>MKLTGKQTWEFENPLFVNSSGTAVGPKEKEGPLGHLFDKSYDEMHCNQKNWEMAERKLMEDAVQSALSKQNLKKEDIDIFLAGDLLNQNVTANYVARHLKIPFLCLFGACSTSMESIAISSALIDGGFAKRALAATSSHNATAERQFRYPTEYGGQKPGTATSTVTGSGAVVLSQQPGGIKITSATVGRVIDLGITDSQDMGSAMAPAAADTIKQHLEDLGRTPDDYDLILTGDLSGVGSPILKDLLKEEGINVGTKHNDCGLMIYTPDQQVFAGGSGCACSAVVTFAHIFKEIEAGRLNRVLVVATGALLSPTIIQQKESIPCIAHGVVFERAERGNALEHHHHH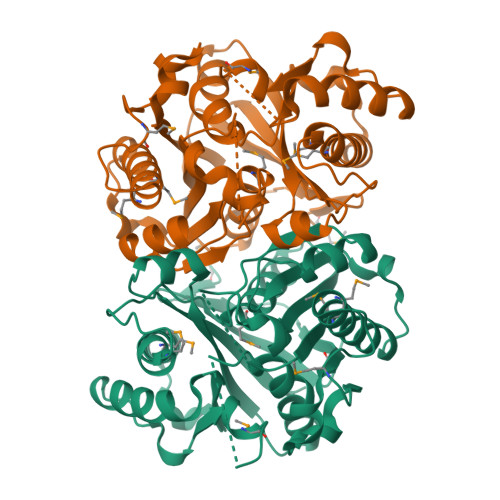H[4x]> GHMIARGKFRSLTLINWNGFFARTFDFDELVTTLSGGNGAGKSTTMAGFVTALIPDLTLLNFRNTTEAGSTSSSRDKGLYGKLKAGVCYAVLETVN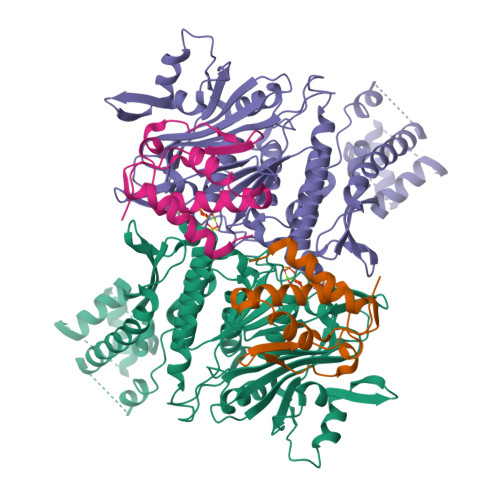SRAQRIITGVRLQQIAGRDKKVDIRPFSLQNVPMTDSVISLFTEQVANKARVLSLNDLKEKFEETAVTFKPYHSITDYHSFMFDLGILPKRLRSSSDRNKFYKLIEASLYGGISSVITKSLRDYLLPENSGVRQAFQDMEAALRENSGGSGGSISAESVANILRKTIQREQNRILQLNQGLQNIAFGQVKGVRLVVNIRDTHSILLNALSDQHEQHKDLFESQKLSFSEALAMLYKRINPHIELGQRMPQTIGEELLDYRNYLDLEVETLRGAYGWMRAESSALSTGEAIGTGMSILLMVVQSWEEESRRMRAKDILPCRLLFLDQAARLDAMSINTLFELCERLDMQLLIAAPENISPERGTTYKLVRKILANQEYVHVVGLKGFG;> MDKNRVFGQRLRQSIQNYFSSPWLLYTAKAEALLDLRDDEAMLNEMEAVGELPMALEYESLTDVQTQIVTAIQAELAHFRNTAQPINLGAVLQEQLARYPQSRHFDVARIIVDQAVKLGMASQDHQAVYPVWQPIDDFSAAVQAHLIDQYDK>[2x]MGSDKIHHHHHHMVR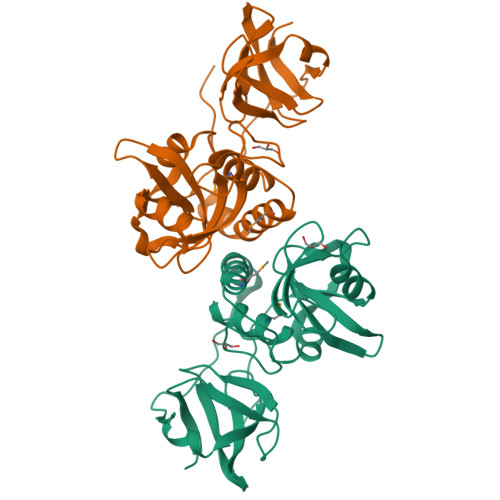LSEAEVQNPKLGEYQCLADLNLFDSPECTRLATQSASGRHLWVTSNHQNLAVEVYLCEDDYPGWLSLSDFDSLQPATVPYQAATFSESEIKKLLAEVIAFTQKAMQQSNYYLWGGTVGPNYDCSGLMQAAFASVGIWLPRDAYQQEGFTQPITIAELVAGDLVFFGTSQKATHVGLYLADGYYIHSSGKDQGRDGIGIDILSEQGDAVSLSYYQQLRGAGRVFKSYEPQRR>MLMPEMDRRRMMMMAGFGALAAALPAPTAWADPSRPAAPAGPTPAPAAPAAATGGLLFHDEFDGPAGSVPDPSKWQVSNHRTPIKNPVGFDRPQFFGQYRDSRQNVFLDGNSNLVLRATREGNRYFGGLVHGLWRGGIGTTWEARIKFNCLAPGMWPAWWLSNDDPGRSGEIDLIEWYGNGTWPSGTTVHANPDGTAFETCPIGVDGGWHNWRVTWNPSGMYFWLDYADGIEPYFSVPATGIEDLNEPIREWPFNDPGYKVFPVLNLAVGGSGGGDP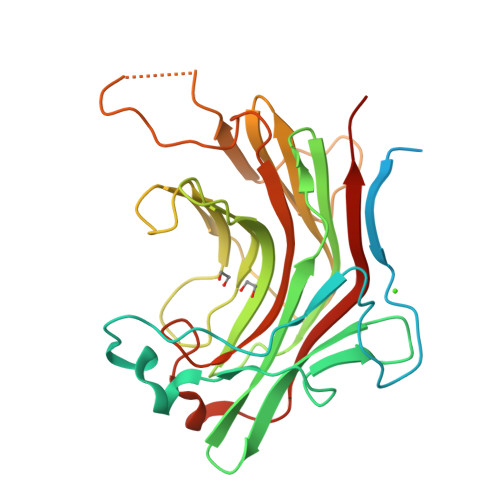ATGSYPQEMLVDWVRVFGSHHHHHH[2x]>FKAERLRVNLRLVINRLKLLEKKKTELAQKARKEIADYLAAGKDERARIRVEHIIREDYLVEAMEILELYCDLLLARFGLIQSMKELDSGLAESVSTLIWAAPRLQSEVAELKIVADQLCAKYSKEYGKLCRTNQIGTVNDRLMHKLSVEAPPKILVERYLIEIAKNYNVPYEPDSVVMAEA[34x];>MEKHLFNLKFAAKELSRSAKKCDKEEKAEKAKIEKAIQKGNMEVARIHAENAIRQKNQAVNFLRMSARVDAVAARVQTAVTMGKVTKSMAGVVKSMDATLK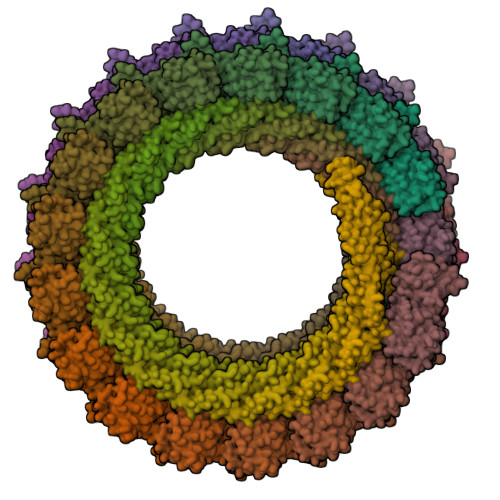TMNLEKISALMDKFEHQFETLDVQTQQMEDTMSSTTTLTTPQNQVDMLLQEMADEAGLD[34x]7-(2-phenylazanylpyrimidin-4-yl)-1,3,4,5-tetrahydro-1-benzazepin-2-one 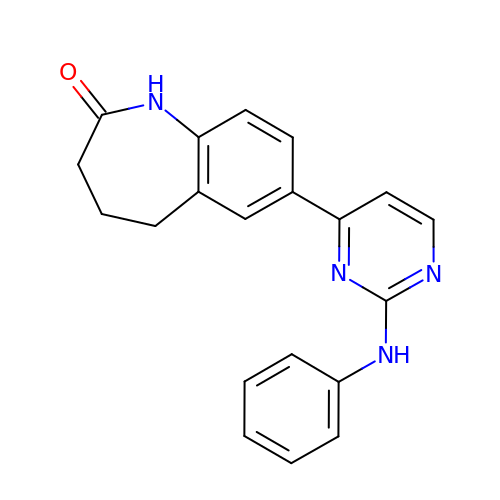| C20 H18 N4 O | YJONEAMNBLRMKD-UHFFFAOYSA-N>[4x]NLYFQGHMVLKLLLELGAERYAEQFAAKCHELGMVMKESAGPGRVPVPVTLQPSMISRGEFGTLCCMQPLWNEAVDNTARNFTFLRDALQETAASDVNFTGKLLNMLQEVYLSGGPFQQLMLGIFRTDYMREGVYDKMLSTTASRWKNVEINTISCSFAGLSPLITEFHQHIAAYLQVLQKARGKEDDDGVENMSWIWGKGNCRLE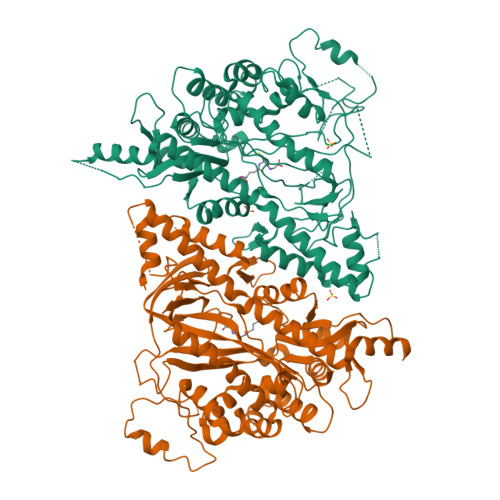RSVSGDVVPKAIADAVRAWVEQQKFASLRASWEQFQQNEVGSGEIHQLGVLDTAPVVLVVVQENERNTADQYALLMRVLEEHRIRFIFRTLQELHLSLKLHSISPEQPPLAVVDGHYPIAVAYFRSTYVPEDFPTDATWAARLSLERSSAIKCPSIPYHLLTFKKLQQLLCDVDRVLVPVAFCGDSDKAGLLQRHFVPQYSLNPKEVGEEAVEKVIHDVLQRPDQFVLKPQLEGGGNLLSGETMVKALKATKEGDPVTYSKVRCEYVVMSRIQFHVSTGSLLARGDVVQLERNMCSEVGIFGVILSAAKGSSVGTNGSSVLFNTFAGYTVRSKPADADDGGVMAGVAALDSLAVVP>STLADLLDHSCTSGSGSGLPFLVQRTVARQITLLECVGKGRYGEVWRGSWQGENVAVKIFSSRDEKSWFRETELYNTVMLRHENILGFIASDMTSRHSSTQLWLITHYHEMGSLYDYLQLTTLDTVSCLRIVLSIASGLAHLHIEIFGTQGKPAIAHRDLKSKNILVKKNGQCCIADLGLAVMHSQSTNQLDVGNNPRVGTKRYMAPEVLDETIQVDCFDSYKRVDIWAFGLVLWEVARRMVSNGIVEDYKPPFYDVVPNDPSFEDMRKVVCVDQQRPNIPNRWFSDPTLTSLAKLMKECWYQNPSARLTALRIKKTLTKIDNS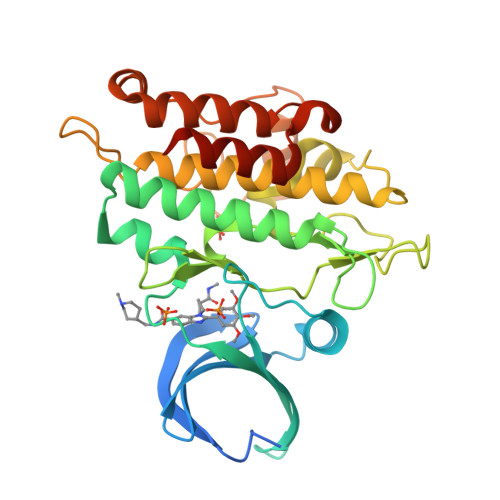LDKLKTDC[2x]>[4x]MASSTFYIPFVNEMGEGSLEKAIKDLNGSGFKNALIVSDAFMNKSGVVKQVADLLKAQGINSAVYDGVMPNPTVTAVLEGLKILKDNNSDFVISLGGGSPHDCAKAIALVATNGGEVKDY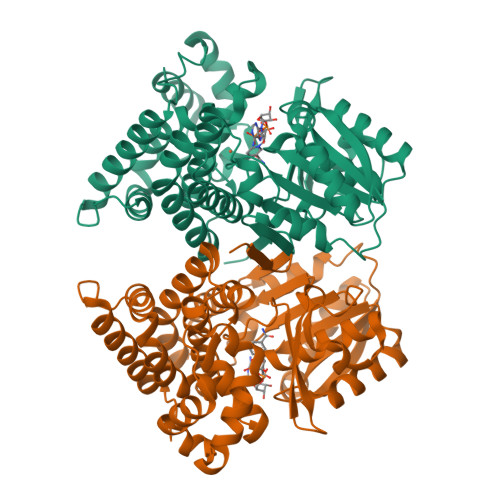EGIDKSKKPALPLMSINTTAGTASEMTRFCIITDEVRHVKMAIVDRHVTPMVSVNDPLLMVGMPKGLTAATGMDALTHAFEAYSSTAATPITDACALKAASMIAKNLKTACDNGKDMPAREAMAYAQFLAGMAFNNASLGYVHAMAHQLGGYYNLPHGVCNAVLLPHVLAYNASVVAGRLKDVGVAMGLDIANLGDKEGAEATIQAVRDLAASIGIPANLTELGAKKEDVPLLADHALKDACALTNPRQGDQKEVEELFLSAF> AFNNNPSSVGAYSSGTYRNLAQEMGKTNIQQKVNSTFDNMFGYNNTQQLYYPYTENGVYKAHYIKAINPDEGDDIRTQGQSWGMTAAVMLNKQEEFDNLWRFAKAYQKNPDNHPDAKKQGVYAWKLKLNQNGFVYKVDEGPAPDGEEYFAFALLNASARWGNSGEFNYYNDAITMLNTIKNKLMENQIIRFSPYIDNLTDPSYHIPAFYDYFANNVTNQADKNYWRQVATKSRTLLKNHFTKVSGSPHWNLPTFLSRLDGSPVIGYIFNGQANPGQWYEFDAWRVIMNVGLDAHLMGAQAWHKSAVNKALGFLSYAKTNNSKNCYEQVYSYGGAQNRGCAGEGQKAANAVALLASTNAGQANEFFN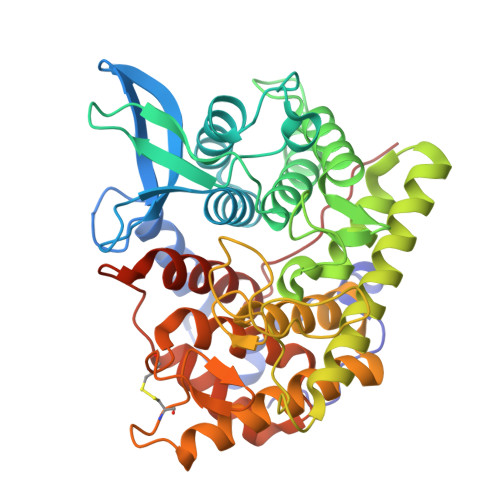EFWSLSQPTGDYRYYNGSLYMLAMLHVSGNFKFYNNTFN> MNYARFITAASAARNPSPIRTMTDILSRGPKSMISLAGGLPNPNMFPFKTAVITVENGKTIQFGEEMMKRALQYSPSAGIPELLSWLKQLQIKLHNPPTIHYPPSQGQMDLCVTSGSQQGLCKVFEMIINPGDNVLLDEPAYSGTLQSLHPLGCNIINVASDESGIVPDSLRDILSRWKPEDAKNPQKNTPKFLYTVPNGNNPTGNSLTSERKKEIYELARKYDFLIIEDDPYYFLQFNKFRVPTFLSMDVDGRVIRADSFSKIISSGLRIGFLTGPKPLI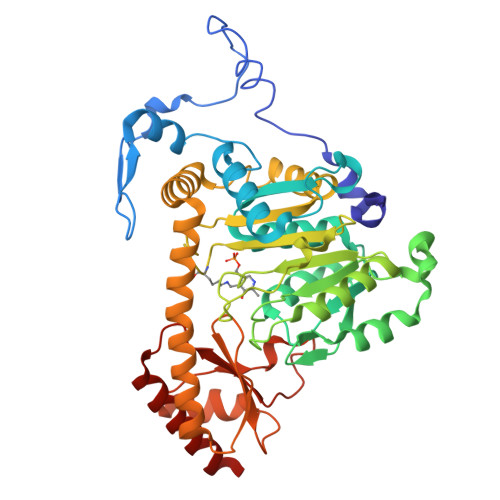ERVILHIQVSTLHPSTFNQLMISQLLHEWGEEGFMAHVDRVIDFYSNQKDAILAAADKWLTGLAEWHVPAAGMFLWIKVKGINDVKELIEEKAVKMGVLMLPGNAFYVDSSAPSPYLRASFSSASPEQMDVAFQVLAQLIKESL>VLGKPQTDPTLEWFLSHCHIHKYPSKSTLIHQGEKAETLYYIVKGSVAVLIKDEEGKEMILSYLNQGDFIGELGLFEEGQERSAWVRAKTACEVAEISYKKFRQLIQVNPDILMRLSAQMARRLQVTSEKVGNLAFLDVTGRIAQTLLNLAKQPDAMTHPDGMQIKITRQEIGQIVGCSRETVGRILKMLEDQNLISAHGKTIVVYGT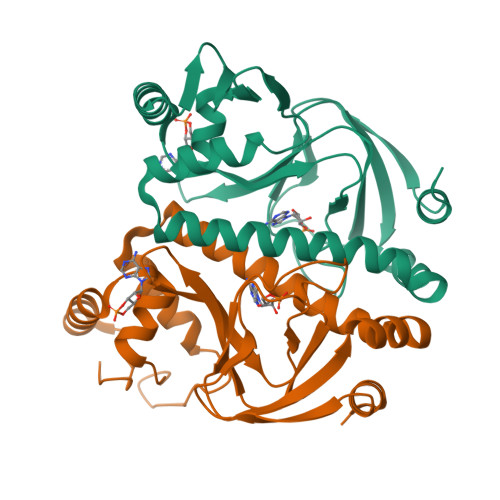R[4x]We characterized CtGH76 from the sordariomycete Chaetomium thermophilum, a member of the Fungi/Bacteria-mixed GH76 subfamily, revealing conserved structural features and functional divergence within the GH76 family. Notably, our structural characterization by X-ray crystallography combined with glycan fragment screening indicated that CtGH76 can recognize GPI-anchors like members of the Dfg5 subfamily but shows a broader promiscuity toward other glycans with central α1,6-mannobiose motifs due to the presence of an elongated glycan-binding canyon. Here, we present the crystal structure of a novel fungal GH76 member from the F/B-mixed subfamily, in complexes with different glycans and glycan fragments. Together with structural bioinformatics, we found that members of the F/B-mixed subfamily act as secreted GHs in glycan degradation, which includes not only α1,6-mannans but also GPI-core glycans. Compared to other GH76 orthologs, our findings demonstrate that CtGH76 features an elongated glycan-binding canyon, adept at accommodating a wider range of complex glycans.

To exclude the residual α1,6-mannasidase activity of CtGH76 under crystal soaking conditions, we generated single-site mutants for its catalytic DD motif. For the active-site mutants D164N and D163N, soaking with α1,6-mannotriose resulted in α1,6-mannobiose binding to subsites −1/−2, alongside with single mannose residues at subsites +3 and −4. However, occupancy of subsite −1 is observed only in the active-site mutants, with slight variations in orientation. For the α1,6-mannobiose complex, the subsite −2 displays a highly conserved binding mode for the mannose moiety, with interactions mediated by a conserved aspartate residue (CtGH76: D268; CtDfg5: D250) that engages the 3- and 4-hydroxyls of mannose. Similarly, subsite −1 features stacking interactions between the mannose pyranose ring and a conserved aromatic residue (CtGH76: W111; CtDfg5: W83). Interestingly, the mannose conformations at subsite −1 differ distinctly between CtGH76 and CtDfg5 complexes. Firstly, CtGH76 favors the β-anomer of the mannose 1-hydroxyl, whereas CtDfg5 prefers the α-anomer. This difference may result from the mutation of D164 in the DD motif to asparagine, causing its sidechain to swivel outward. Secondly, the mannosyl moiety in CtDfg5 adopts a regular 4C1 boat conformation, while in CtGH76, the pyranose ring is distorted into an OS2-like conformation. The α1,6-mannobiose at subsite −1 adopts an OS2 conformation in CtGH76, resembling a strained substrate, with a subtle shift likely caused by the active site mutation D164N.

> MAGIADLTAALASADRNRVTRVEAMRRSPTTISLSTLGALSALWGILYFMTCSGRNSRGVLADASSGMLQTRQSDSESLNSTGLAQAAINGLNARFYESSNARWSSDEPWWISGVALTMVIEYMRRSGSKEYLDQVEDVIEVQRQPLSWWPSGEGEFRADATDNTGWWALAMVRMYDLTGNEDYLNISIKDEAYMRQWWTDTECGGGLYVDIQDLTYKNAIANELYLKLVASLANRAPNATIYLDRAQQAWTWFLGSGMINGVNLINDGLARDSNTGSCYNNRLPVWTYNQGVILGALVELYHATKDESYLLSAQAIADAVLSPSNGLTSSSGVLTETCEGSDSCNQDQQVFKGVFALNLAELGDAVAGASSDPDAGQDYREYLDTNMQSMYANDRSEIVPTLFDSSTGDLYDVSWSGPFRNATMPKQASAIGLYVANI> GSMVPPPENVRMNSVNFKNILQWESPAFAKGQLTFTAQYLSYRIFQDKCMQTTLTECDFSSLSKYGDHTLRVRAEFADEHSDWVQITFCPVDDTIIGPPGMQVEVLADSLHMRFLAPKIENEYETWTMKDMYNSWTYNVQYWKQGTDEKFQITPQYDFEVLRNLEPRTTYCVQVRGFLPDRNKAGEWSEPVCEQTTHDETVPSAAAHHHHHH;> RPRLAPPQNVTLLSQNFSVYLTWLPGLGNPQDVTYFVAYQSSPTRRRWREVEECAGTKELLCSMMCLKKQDLYNKFKGRVRTVSPSSKSPWVESEYLDYLFEVEPAPPVLVLTQTEEILSANATYQLPPCMPPLDLKYEVAFWKEGAGNKTLFPVTPHGQPVQITLQPAASEHHCLSARTIYTFSVPKYSKFSKPTCFLLEVPEANAAA;> GGGSGAAAPRRCLLSHYRSLEPRTLAAAKALRDRYEEEALSWGQRNCSFRPRRDPPRPSSCARLRHVARGIADAQAVLSGLHRSELLPGAGPILELLAAAGRDVAACLELARPGSSRKVPGAQKRRHKPRRADSPRCRKASVVFNLLRLLTWELRLAAHSGPCLAAAHHHHHHHH

When they were initially discovered, type III interferons (IFNλ1-3) were structurally and evolutionarily classified as members of the IL-10 superfamily of cytokines. Further investigation, though, revealed that they are functionally interferons (IFNs) with distinct roles in mucosal and innate immunity. While predicted to be structurally similar to IFNλ1-3, IFNλ4 shares only 28% amino acid sequence identity with its closest relative IFNλ3 and has a distinct biochemical composition resulting in IFNλ4 being one of the most positively-charged known cytokines (pI = 11.3). We next use protein engineering to overcome the affinity limitation for structural determination of the ternary IFNλ cytokine-receptor complex and determine the 72 kilodalton (kDa) structures of IFNλ4 as well as IFNλ3 in complex with IFNλR1 and an affinity-matured IL10Rβ via cryogenic electron microscopy (cryoEM).

A The structure of the IFNλ4 (red) ternary complex elucidates the mechanism of IFNλR1 (gray) and IL10Rβ-A3 (gold) engagement. IFNλ4 engages IFNλR1 with higher surface area and has fewer polar contacts with IL10Rβ. However, IFNλ4 forms more polar contacts at this interface, with eight compared to four for IFNλ3, featuring unique involvement of the Ser185 residue on IFNλR1 forming three hydrogen bonds with residues Pro37, Arg38, and Ala41. While the overall topology of this interface is similar between IFNλR1 and the IFNλs, these chains find themselves in closer proximity to IFNλR1 on IFNλ4, leading to a 38% higher buried surface area (BSA) at the IFNλ4:IFNλR1 interface (1740.7 Å2) compared to IFNλ3:IFNλR1 (1260.1 Å2). Ultimately this leads to an affinity of 191 nM between IFNλ4 and IFNλR1 as measured by surface plasmon resonance (SPR), more than 4-fold higher affinity than the previously published 850 nM interaction between IFNλ3 and IFNλR127. While Tyr140 remains in largely the same place, the Trp143 residue in IFNλ4 is in a flipped orientation compared to IFNλ3 but in both structures is buried at the interface. There is the same observed “pinch” on Helix A of IFNλ4 formed by Tyr140 and Trp143 as with IFNλ3-H11, with Tyr140 forming a hydrogen bond with Arg38 on IFNλ4 and Trp143 forming a hydrogen bond with the backbone oxygen of Leu35. Comparison of the structures highlights differences in receptor engagement and reveals a distinct 12-degree rotation in overall receptor geometry, providing a potential mechanistic explanation for differences in cell signaling, downstream gene induction, and antiviral activities. During structural refinement, however, we were unable to resolve the structure of Helix E of IFNλ4. While this region of the protein is uninvolved in receptor engagement, molecular modeling reveals that this highly basic region of IFNλ4 containing the amino acid sequence KRRHKPRR is predicted to lack secondary structure unlike the corresponding region of IFNλ3, breaking from the structural symmetry of the two proteins.> KDIQLLNVSYDPTRELYEQYNKAFSAHWKQETGDNVVIDQSHGGSGKQATSVINGIEADTVT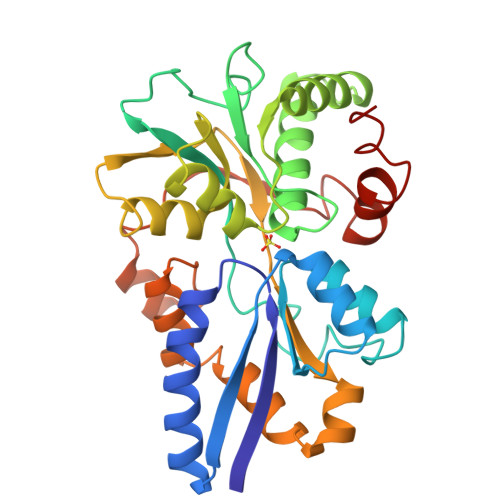LALAYDVNAIAERGRIDKNWIKRLPDDSAPYTSTIVFLVRKGNPKQIHDWNDLIKPGVSVITPNPKSSGGARWNYLAAWGYALHHNNNDQAKAEDFVKALFKNVEVLDSGARGSTNTFVERGIGDVLIAWENEALLATNELGKDKFEIVTPSESILAEPTVSVVDKVVEKKDTKAVAEAYLKYLYSPEGQEIAAKNFYRPRDADVAKKYDDAFPKLKLFTIDEVFGGWAKAQKDHFADGGTFDQISKR>ATDTLANEDCFRHESLVPNLDYERFRGSWIIAAGTSEALTQYKCWIDRFSYDDALVSKYTDSQGKNRTTIRGRTKFEGNKFTIDYNDKGKAFSAPYSVLATDYENYAIVEGCPAAANGHVIYVQLRMTLRRFHPKLGDKEMLQHYTLDQVNQNKK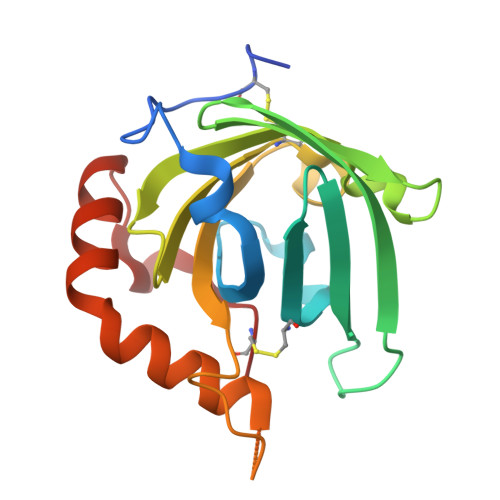AIEEDLKHFNLKYEDLHSTCH[2x]>MSSGNAKIGHPAPSFKATAVMPDGQFKDISLSDYKGKYVVFFFYPLDFTFVSPTEIIAFSDRAEEFKKLNCQVIGASVDSHFCHLAWINTPKKQGGLGPMNIPLVSDPKRTIAQDYGVLKADEGISFRGLFIIDDKGILRQITINDLPVGRSVDEILRLVQAFQFTDKHGEVCPAGWKPGSDTIKPDVNKSKEYFSKQK[1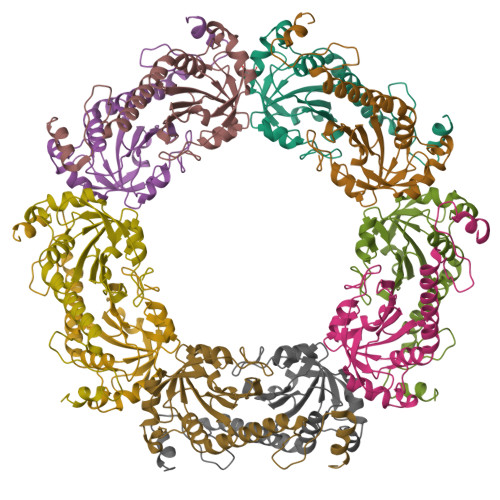0x]>GPMGTDWPVYHRIDGPIVMIGFGSIGRGTLPLIERHFAFDRSKLVVIDPSDEARKLAEARGVRFIQQAVTRDNYRELLVPLLTAGPGQGFCVNLSVDTSSLDIMELARENGALYIDTVVEPWLGFYFDPDLKPEARSNYALRETVLAARRNKPGGTTAVSCCGANPGMVSWFVKQALVNLAADLGVTGEEPTTREEWARLAMDLGVKGIHIAERDTQRASFPKPFDVFVNTESVEGFVSEGLQPAELGWGTFERWMPDNARGHDSGCGAGIYLLQPGANTRVRSWTPTAMAQYGFLVTHNES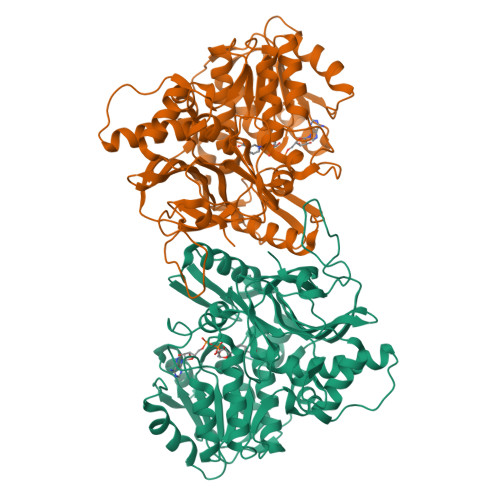ISIADFLTVRDAAGQAVYRPTCHYAYHPCNDAVLSLHEMFGSGKRQSDWRILDETEIVDGIDELGVLLYGHGKNAYWYGSQLSIEETRRIAPDQNATGLQVSSAVLAGMVWALENPNAGIVEADDLDFRRCLEVQTPYLGPVVGVYTDWTPLAGRPGLFPEDIDTSDPWQFRNVLVRD[2x]>[2x]ASLTEIEH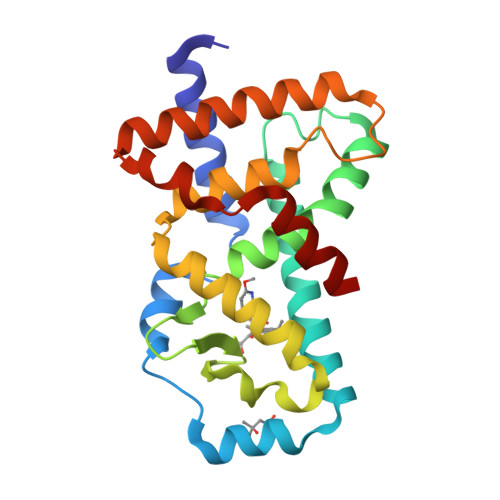LVQSVCKSYRETCQLRLEDLLRQRSNIFSREEVTGYQRKSMWEMWERCAHHLTEAIQYVVEFAKRLSGFMELCQNDQIVLLKAGAMEVVLVRMCRAYNADNRTVFFEGKYGGMELFRALGCSELISSIFDFSHSLSALHFSEDEIALYTALVLINAHRPGLQEKRKVEQLQYNLELAFHHHLCKTHRQSILAKLPPKGKLRSLCSQHV>MSKPDRVVLIGVAGDSGCGKSTFLNRLADLFGTELMTVICLDDYHSLDRKGRKEAGVTALDPRANNFDLMYEQVKALKNGETIMKPIYNHETGLIDPPEKIEPNRIIVIEGLHPLYDERVRELLDFSVYLDIDDEVKIAWKIQRDMAERGHSYEDVLASIEARRPDFKAYIEPQRGHADIVIRVMPTQLIPNDTE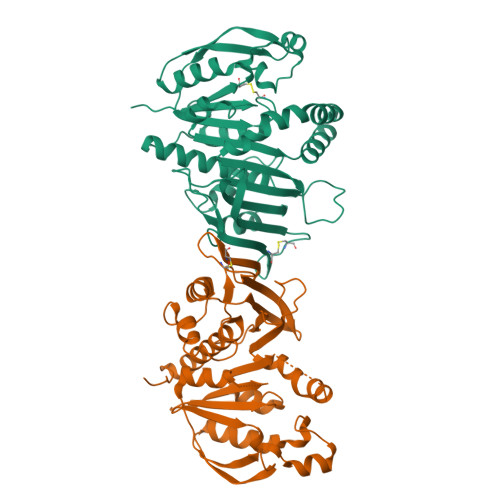RKVLRVQLIQREGRDGFEPAYLFDEGSTIQWTPCGRKLTCSYPGIRLAYGPDTYYGHEVSVLEVDGQFENLEEMIYVEGHLSKTDTQYYGELTHLLLQHKDYPGSNNGTGLFQVLTGLKMRAAYERLTSQAAPVAASV[2x]5-(1-methyl-1H-imidazol-4-yl)-2-[(1-{[4-(trifluoromethoxy)phenyl]acetyl}piperidin-4-yl)oxy]benzamide | C25 H25 F3 N4 O4 | 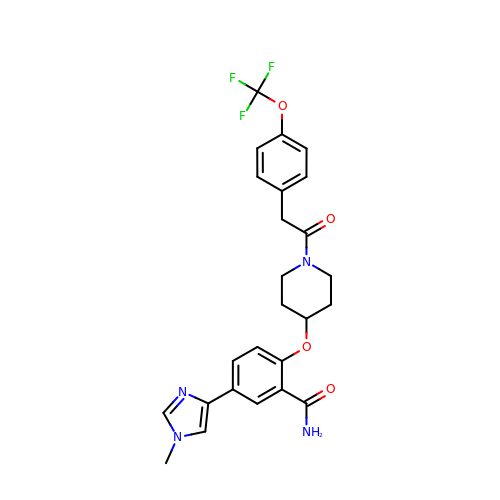VXJAFFGXYYHGQN-UHFFFAOYSA-N>[4x]MKITNPVLKGFNPDPSICRAGEDYYIAVSTFEWFPGVQIHHSKDLVNWHLVAHPLQRVSQLDMKGNPNSGGVWAPCLSYSDGKFWLIYTDVKVVDGAWKDCHNYLVTCETINGDWSEPIKLNSSGFDASLFHDTDGKKYLLNMLWDHRIDRHSFGGIVIQEYSDKEQKLIGKPKVIFEGTDRKLTEAPHLYHIGNYYYLLTAEGGTRYEHAATIARSANIEGPYEVHPDNPILTSWHDPGNPLQKCGHASIVQTHTDEWYLAHLTGRPIHPDDDSIFQQRGYCPLGRETAIQKLYWKDEWPYVVGG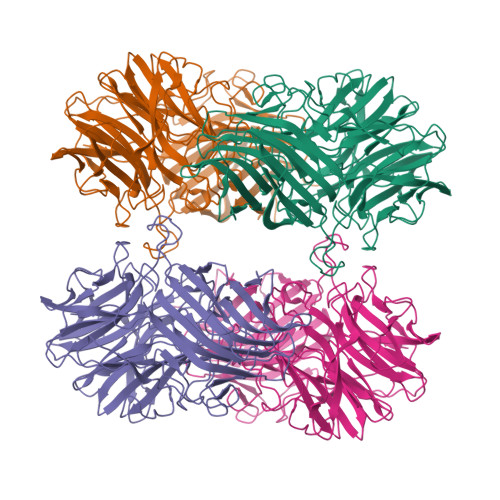KEGSLEVDAPSIPETIFEATYPEVDEFEDSTLNINFQTLRIPFTNELGSLTQAPNHLRLFGHESLTSTFTQAFVARRWQSLHFEAETAVEFYPENFQQAAGLVNYYNTENWTALQVTHDEELGRILELTICDNFSFSQPLNNKIVIPREVKYVYLRVNIEKDKYYYFYSFNKEDWHKIDIALESKKLSDDYIRGGGFFTGAFVGMQCQDTGGNHIPADFRYFRYKEK>[2x]MNKHTNLVTSSFNLTKPMKSFIRRNGLRVQESVTDETDFVILGSPPLRRTHKFLLA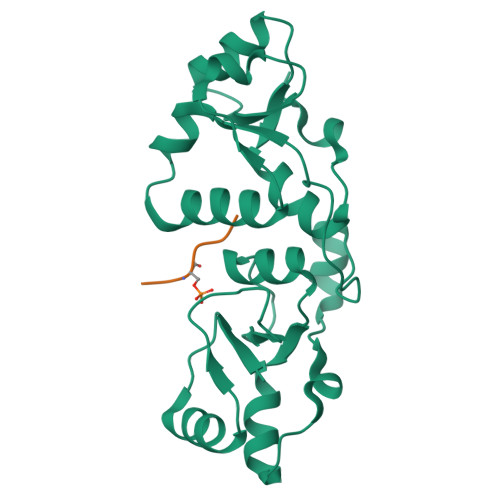TSLGIPLVSSQYLTDCIKSGKVLDFRSYKYKDEEAEAKWGFRLDDIHRRTCFNGKRLYITKAIRDSMVGDSIHGLYSILETSGAEIVGDIKRAQEKDTIILAQPDNDQEGRNMSATGLNVYKIELVALSILRDRIDFDEFLID;>SGRTGKPSQEL[2x]> MVVSLRRFHSYANSSRGGATTCLITGGGKGHFALTVSTRGRFYRPLVDDGINLWRRRMGRIHKGWRTWEYQHTRPDPRPFPDPPVNDYFGRSRIWNPIACKLGYVRKKADEWGWPNKPPPPTGLRYSQEFFPFFFERYFPDAEVRLLLDSVLNNETKRPVFQIPCSMSKVELVNYLKNIYGIDNVVRVEVRNRRGRRYKN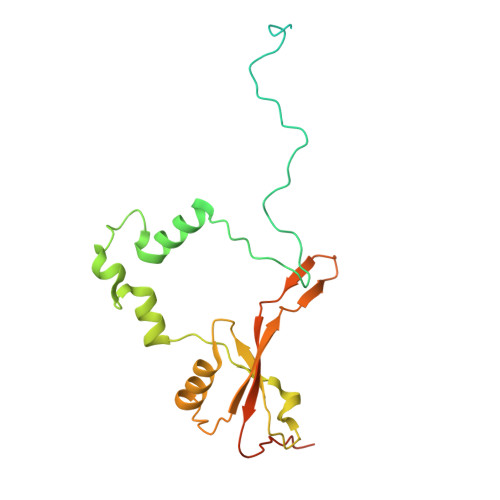EVGEIKMMDDYKVAVVELDTPVSVELKQIKGTEDTSDNRPQERITQ>[2x]MEDPYIWMENLEDERVLKIIEEENKRFREFIGELSDKLFPEVWEQFSQPTIGMARITKKGIIASYSEKDRVVIKWFNGDVIVDSKELEREVGDEVLLQGFTTDEEGEKLAYSFSIGGADEGITRIIDLKTGEVIEEIKPSIWNITFLKDGYYFTRFYRKEKTPDGVNPPAARMFWKDREGERMVFGEGLTSGYFMSIRKSSDGKFAIVTLTYGWNQGEVYIGPIDNPQEWKKVYSASVPVEAIDVVNGKLYILTKEGKGLGKIIAIKNGKIDEVIPEGEFPLEWAVIVRDKILAGRLVHASYKLEVYTLNGEKIKEITFDVPGSLYPLDKDEERVLLRYTSFTIPYRLYEFKDDLRLI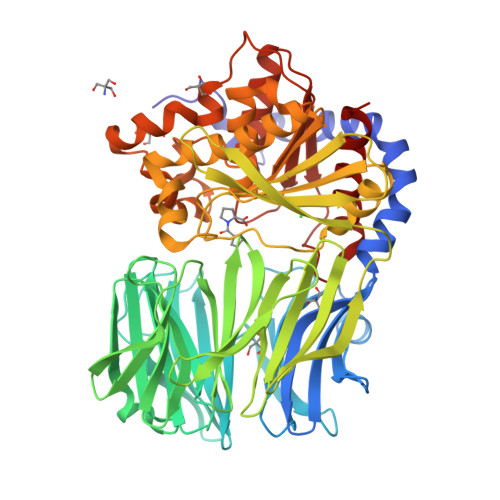EERKVEGEFRVEEDFATSKDGTKVHYFIVKGERDEKRAWVFGYGGFNIALTPMFFPQVIPFLKRGGTFIMANLRGGSEYGEEWHRAGMRENKQNVFDDFIAVLEKLKKEGYKVAAWGRSNGGLLVSATLTQRPDVMDSALIGYPVIDMLRFHKLYIGSVWIPEYGNPEDPKDREFLLKYSPYHNVDPKKKYPPTLIYTGLHDDRVHPAHALKFFMKLKEIGAPVYLRVETKSGHMGASPETRARELTDLLAFVLKTLS> THWFHRNPLKATAPVSFNYYGVVTGPSASKICNDLRSSRARLLELFTDLSCNPEMMKNAADSYFSLLQGFINSLDESTQESKLRYIQNFKWTDTLQGQVPSAQQDAVFELISMGFNVALWYTKYASRLAGKENITEDEAKEVHRSLKIAAGIFKHLKESHLPKLITPAEKGRDLESRLIEAYVIQCQ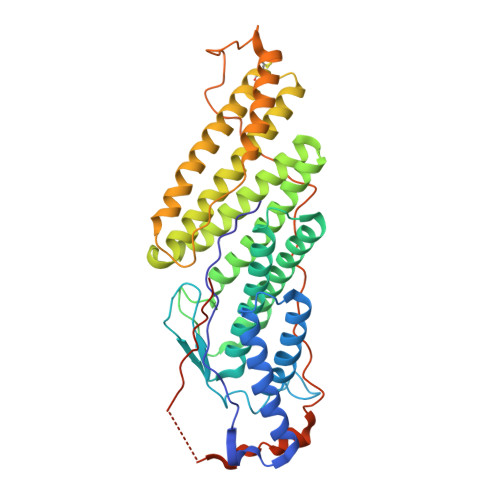AEAQEVTIARAIELKHAPGLIAALAYETANFYQKADHTLSSLEPAYSAKWRKYLHLKMCFYTAYAYCYHGETLLASDKCGEAIRSLQEAEKLYAKAEALCKEYGETKGPGPTVKPSGHLFFRKLGNLVKNTLEKCQRENGFIYFQKIPTEAPQLELKANYGLVEPIPFEFPPTSVQWTPETLAAFDLTKRPKDDSTKPKPEEEVKPVKEPDIKPQKDTGCYIS> MGPFDPEEMLFIFTRCMEDNLEDGANRL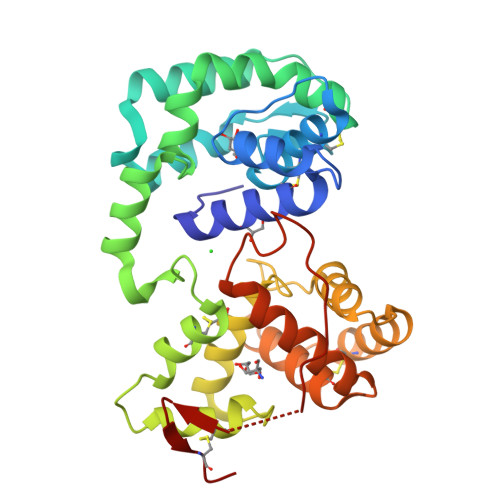PMLAKWKEWINEPVDSPATQCFGKCVLVRTGLYDPVAQKFDASVIQEQFKAYPSLGEKSKVEAYANAVKQLPSTNNDCAAVFKAYDPVHKAHKDTSKNLFHGNKELTKGLYEKLGKDIRQKKQSYFEFCENKYYPAGSDKRQQLCQIRQYTVLDDALFKEHTDCVMKGIRYITKDNQLDVEEVKRDFKLVNKDTKALEEVLNDCKSKEPSNAKEKSWHYYKCLVESSVKDDFKEAFDYREVRSQIYAFNLPKNQAYSKPAVQSQVMEIDGKQCPQ> PGSEDENKLLEACIFKNNELLKNIQDVQSQISKIGLKDPTVPAVKHRKKSLIRLDKVLDEYEEEKRHLQEMANSLPHFKDGREKTVNQQCQNTVVLWENTKALVTECLEQCGRVLELLKQYQNFKSILTTLIQKEESVISLQASYMGKENLKKRIAEIEIVKEEFNEHLEVVDKINQVC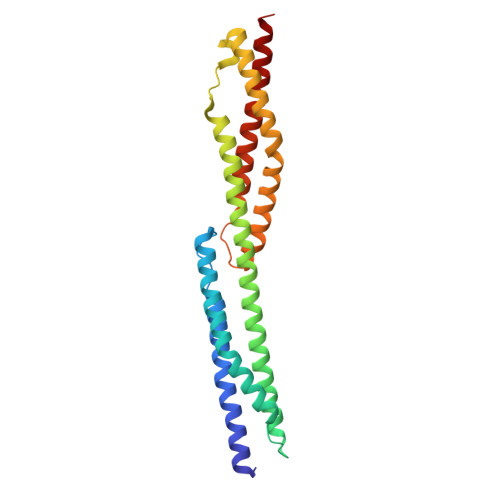KNLQFYLNKMKTFEEPPFEKEANIIVDRWLDINEKTEDYYENLGRALALWD>MAKTQAEINKRLDAYAKGTVDSPYRVKKATSYDPSFGVMEAGAIDADGYYHAQCQDLITDYVLWLTDN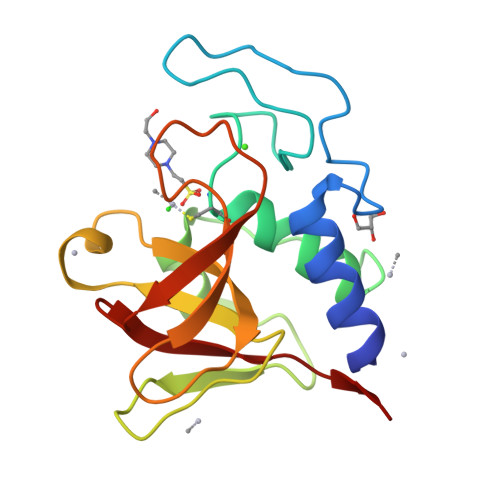KVRTWGNAKDQIKQSYGTGFKIHENKPSTVPKKGWIAVFTSGSYEQWGHIGIVYDGGNTSTFTILEQNWNGYANKKPTKRVDNYYGLTHFIEIPVKA[4x]> MTIDINKLKEELGLGDLAKSLEGLTAAQKAQEAERMRKEQEEKELARMNDLVSKAVGEDRKRLEEALELVKSLDEKSKKSNELFAQTVEKQQETIVGLQDEIKSLLTAREGRSFVGDSVAKALYGTQENFEDEVEKLVLLSYVMEKGVFETEHGQRHLKAVNQSSSVEVSSESYETIFSQRIIRDLQKELVVGALFEELPMSSKILTMLVEPDAGKATWVAASTYGTDTTTGEEVKGALKEIHFSTYKLAAKSFITDETEEDAIFSLLPLLRKRLIEAHAVSIEEAFMTGDGSGKPKGLLTLASEDSAKVVTEAKADGSVLVTAKTISKLRRKLGRHGLKLSKLVLIVSMDAYYDLLEDEEWQDVAQVGNDSVKLQGQVGRIYGLPVVVSEYFPAKANSAEFAVIVYKDNFVMPRQ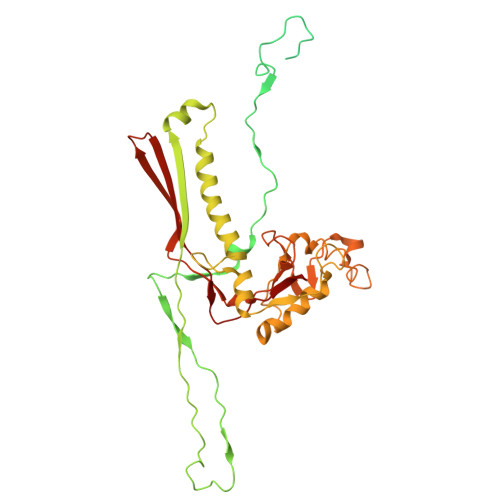RAVTVERERQAGKQRDAYYVTQRVNLQRYFANGVVSGTYAAS> MNVQDRRRLLGPAAAKPMAFSNTTTHVPEKKSTDLTPKGNESEQELSLHTGF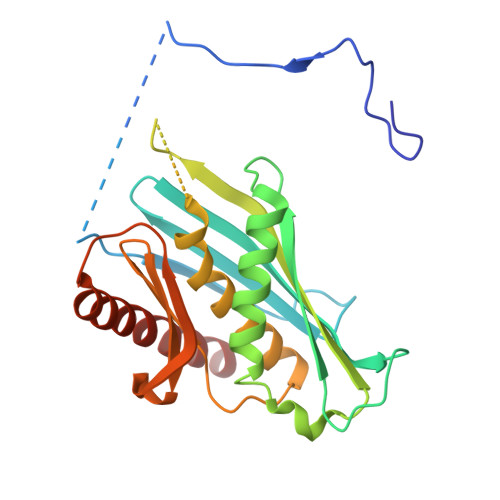IENCNGSALVEARSLGHQTSLISAVYGPRSIRGSFTSQGTISIQLKNGLLEKYNTNELKEVSSFLMGIFNSVVNLSRYPKSGIDIFVYLTYDKDLTNNPQDDDSQSKMTSSQISSLIPHCITSITLALADAGIELVDMAGAGEANGTVVSFIKNGEEIVGFWKDDGDDEDLLECLDRCKEQYNRYRDLMISCLMNQET1-[3-(trifluoromethyl)phenyl]urea | C8 H7 F3 N2 O | 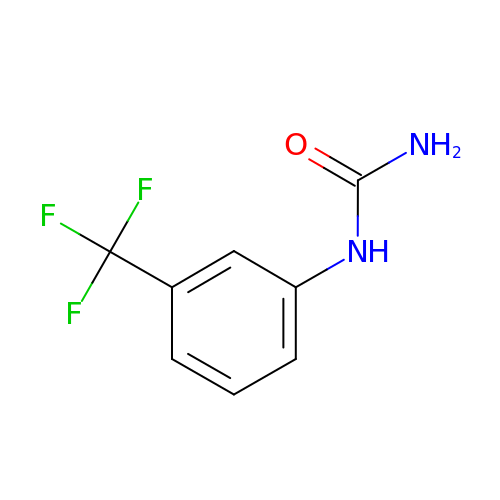FQEIBEOBXKJAMZ-UHFFFAOYSA-N>[2x]MAHHHHHHGHHHQ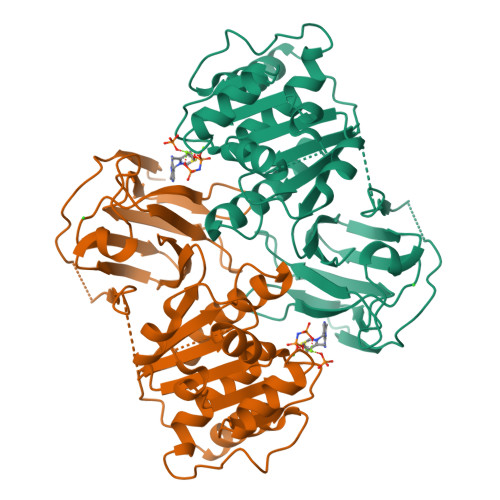LSEDSELIEQVIEQPDSLIISPPSDSSSSSYNHIQPFVYLESTATTQTNHNVLLILNQKITIDLISLWKKCEIIVCADGGANSLYEYFNDNNHHHHHENLQRSDYIPDYIVGDFDSISPDVKTYYESHGSKIIRQSSQYYNDFTKSIHCIQLHYQLNHTKENWFESIDEVDGLAKLWNGLNNSSDVVVDIDITIYVLNAIGGRFDQTVQSINQLYIMNEDYPKVTVFFITTNDIIFLLKKGVNYISYKNRLMFHKDNGSSPTPTCGLLPLSNKTPIILNSYGLKYDMRNWKTEMLGQVSSSNRISGETGFIVECSDDIVMNIEIDVQLDGDLEAA>[2x]GHMVSCSAPGKIYLFGEHAVVYGETAIACAVELRTRVRAELNDSITIQSQIGRTGLDFEKHPYVSAVIEKMRKSIPINGVFLTVDSDIPVGSGLGSSAAVTIASIGALNELFGFGLSLQEIAKLGHEIEIKVQGAASPTDTYVSTFGGVVTIPERRKLKTPDCGIVIGDTGVFSSTKELVANVRQLRESYPDLIEPLMTSIGKISRIGEQLVLSGDYASIGRLMNVNQGLLDALGVNILELSQLIYSARAAGAFGAKITGAGGGGCMVALTAPEKCNQVAEAVAGAGGKVTITKPTEQGLKVD

A key regulatory step in the mevalonate pathway is the ATP-dependent phosphorylation of (R)-mevalonate to (R)-5-phosphomevalonate catalyzed by the enzyme mevalonate kinase (MK), a member of the galacto-/homoserine/mevalonate/phosphomevalonate (GHMP) kinase family. Distributed widely across eukaryotes, bacteria, and archaea, the mevalonate pathway consists of seven enzymes that convert three molecules of acetyl-CoA to isopentenyl pyrophosphate (IPP) and dimethylallyl pyrophosphate (DMAPP), the isomeric, five-carbon precursors to all steroids and isoprenoids. Each MK monomer consists of two domains, where the active site lies on a surface cleft at the interdomain interface. To shed greater light onto the mechanism of MK and to further investigate archaeal MK in particular, we determined the X-ray structures of MmMK bound with the substrate mevalonate and with the product 5-phosphomevalonate.

In particular, the structure of 5-phosphomevalonate represents the first crystal structure of any MK bound with its product. In the 5-phosphomevalonate-bound MmMK structure, the mevaldyl moiety of the product is located in a similar position as in the mevalonate-bound MmMK structure, displaying the same lack of direct contacts with the enzyme. The phosphate group, however, interacts with Asp138, a catalytically important residue discussed in greater detail below. In comparing the mevalonate- and phosphomevalonate-bound structures, there are no significant changes in the protein backbone and residues in the active site also do not display significantly altered orientations, indicating that the transformation of the substrate to the product does not trigger major protein rearrangements. Our structures of mevalonate- and 5-phosphomevalonate-bound MmMK align very well with each other, with root-mean-square deviation for Cα atoms (rmsd) of 0.18 Å, indicating no significant structural differences between the substrate- and the product-bound enzyme. Once the phosphoryl group is transferred to form 5-phosphomevalonate, our structure of product-bound MmMK depicts few structural alterations upon product formation. Although we cannot assign protonation states of all ionizable groups, our structures suggest that the negatively charged phosphate group of the product now interacts with the now-protonated Asp138, consistent with its proposed role in deprotonation described above. Notably, fewer ordered water molecules appear to be bound in this region of our 5-phosphomevalonate MmMK structure. Although the poorer resolution of the 5-phosphomevalonate-bound MmMK structure may itself hinder the visualization of water molecules, the presence of the phosphate group would necessarily displace water molecules that were present in this region of the mevalonate-bound structure.> NTETKTEKTVKDADQNIQDAYTYTIKADAPTWGKDKKLTAFRFEDELDKRLDFQKVTEVKAGDTVLGTSDYTVNDPATDGNKLVVTLTDEGLKKVKSGDKMSLTFEVKRKEVGNTTELKNRADVIFNNPNTDKEVKNKTNEVVTYHGKLKVVKKDGKEAGKVLKGAEFELYQCTSAAVLGKGPLTVDGVKKWTTGDDGTFTIDGLHVTDFEDGKEAAPATKKFCLKETKAPAGYALPDPNVTEIEFTRAKISEKDKFEGDDEVTLVSEIKNIKQGT

SpaD, the subject of this report, is the major pilin protein that forms the polymeric backbone, or shaft, of one of the three types of pilus expressed by the human pathogen C. diphtheriae. SpaD is an elongated molecule of ∼125 Å in length built from three tandem domains with Ig-type folds. As in some of the other Gram-positive major pilins, these three domains comprise a single CnaA-type domain flanked by two CnaB-type domains. Two crystal structures, of the full-length three-domain protein at 2.5 Å resolution and of a two-domain (D2-D3) construct at 1.87 Å resolution, show that each of the three Ig-like domains contains a single Lys–Asn isopeptide-bond cross-link, assumed to give mechanical stability as in other such pili.

We therefore sought to prepare a stable truncated fragment of SpaD that could be crystallized and used to solve the structure of the full-length protein by molecular replacement. This was achieved by partial trypsin digestion of the full-length selenomethionine-labelled form of SpaD (SeMet SpaD). Mass spectrometry confirmed the mass of the resulting product to be 30 456.00 Da, corresponding to residues 180–455. This truncated form of SpaD (SeMet SpaDtryp) was crystallized in space group P212121 and its structure was solved by single-wavelength anomalous diffraction (SAD) methods from in-house data collected at a wavelength of 1.5418 Å, utilizing the signals from one Se atom, one Ca2+ ion and two S atoms (from a disulfide bond). The calcium ion was also used during phasing of SeMet SpaDtryp and gave rise to an anomalous signal consistent with that expected from calcium at an X-ray wavelength of 1.5418 Å. In contrast, domains D2 and D3 are almost linearly connected, with strands β17 and β18 running through the length of both domains. The D3 domain contains a calcium-binding site formed within a loop between strands β23 and β24.>MQAAADRRTVEKTWKLMDKVVRLCQNPKLQLKNSPPYILDILPDTYQHLRLILSKYDDNQKLAQLSENEYFKIYIDSLMKKSKRAIRLFKEGKERMYEEQSQDRRNLTKLSLIFSHMLAEIKAIFPNGQFQGDNFRITKADAAEFWRKFFGDKTIVPWKVFRQCLHEVH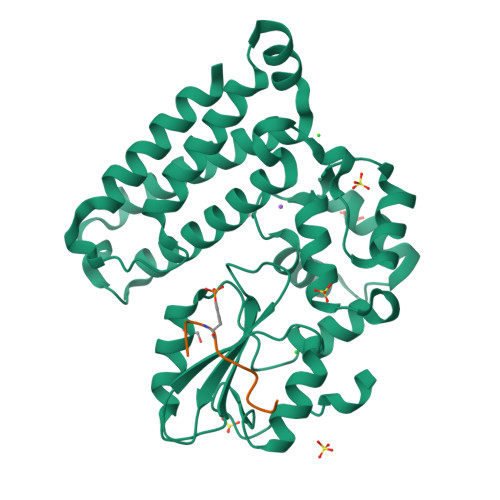QISSGLEAMALKSTIDLTCNDYISVFEFDIFTRLFQPWGSILRNWNFLAVTHPGYMAFLTYDEVKARLQKYSTKPGSYIFRLSCTRLGQWAIGYVTGDGNILQTIPHNKPLFQALIDGSREGFYLYPDGRSYNPDLTGLAENLYFQ[2x];>LQRYSSDPTGA[2x]> MVEYRAEVGQNAYLPCF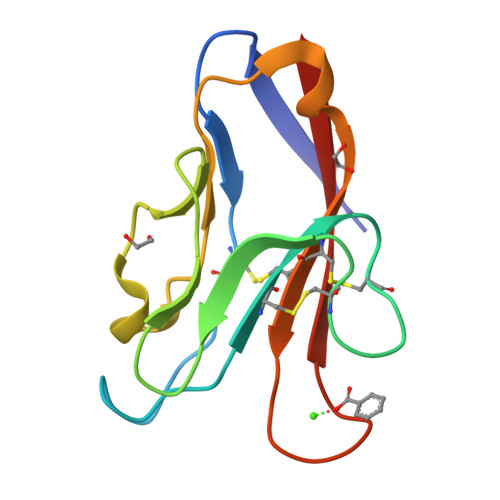YTPAAPGNLVPVCWGKGACPVFECGNVVLRTDERDVNYWTSRYWLNGDFRKGDVSLTIENVTLADSGIYCCRIQIPGIMNDEKFNLKLVIK> WKLPSVTV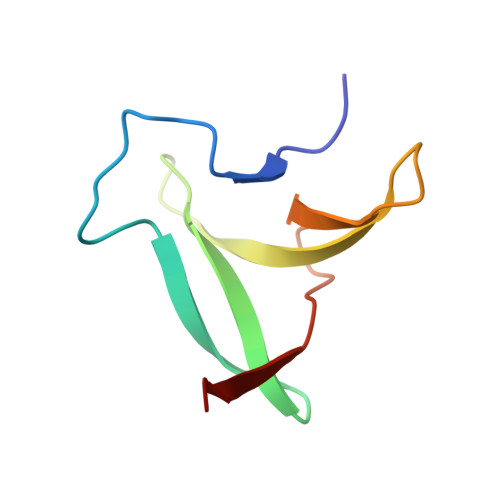GNPKVSVFGGPFKIEEGKSGYKDVYSSSKGRDLDDGIEVNKKKEKRLVVKDGNPFIIRFKKSG>[4x]GPKLREV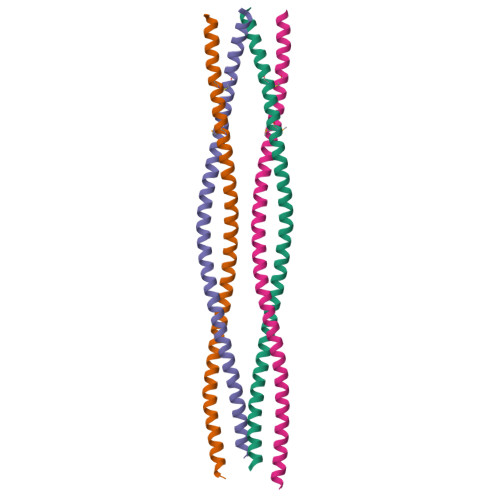KYELDTKVSELSHKLGSSEGSNRSLEEETARLRSLNQQLSSSKHELEIQLNEAKAKVLALDEKAQSQGDVIEQQRGRLRDMEAALRQTEQRCADLRDTLASAEGRAKEA> QILPIRFQEHLQLQNLGINPANIGFSTLTMESDKFICIREKVGEQAQVVIIDMNDPSNPIRRPISADSAIMNPASKVIALKAGKTLQIFNIEMKSKMKAHTMTDDVTFWKWISLNTVALVTDNAVYHWSMEGESQPVKMFDRHSSLAGCQIINYRTDAKQKWLLLTGIS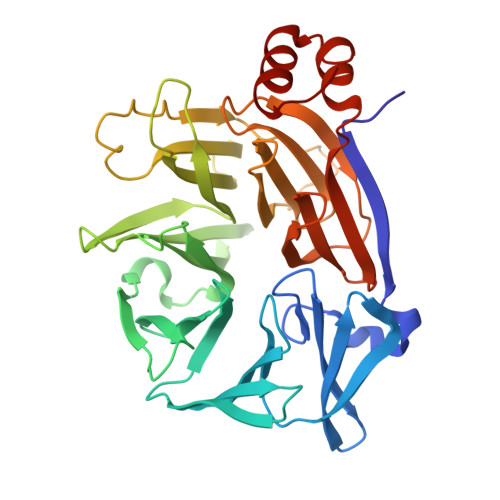AQQNRVVGAMQLYSVDRKVSQPIEGHAASFAQFKMEGNAEESTLFCFAVRGQAGGKLHIIEVGTPPTGNQPFPKKAVDVFFPPEAQNDFPVAMQISEKHDVVFLITKYGYIHLYDLETGTCIYMNRISGETIFVTAPHEATAGIIGVNRKGQVLSVCVEEENIIPYITNVLQNPDLALRMAVRNNLAG>AKPQIPKDKSKVAGYIEIPDADIKEPVYPGPATPEQLNRGVSFAEENESLDDQNISIAGHTFIDRPNYQFTNLKAAKKGSMVYFKVGNETRKYKMTSIRDVKPT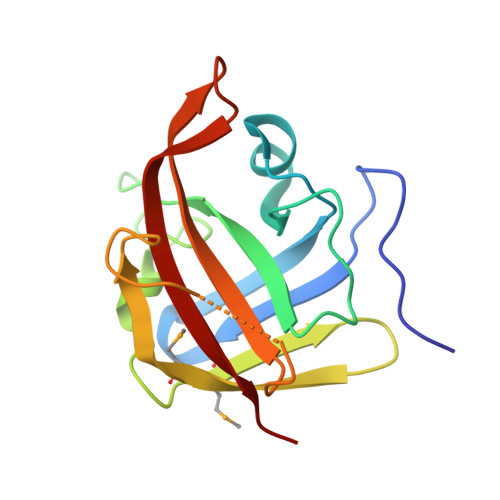DVGVLDEQKGKDKQLTLITADDYNEKTGVWEKRKIFVATEVK[3x]>MSKATYKERAATHPSPVAAKLFNIMHEKQTNLCASLDVRTTKELLELVEALGPKICLLKTHVDILTDFSMEGTVKPL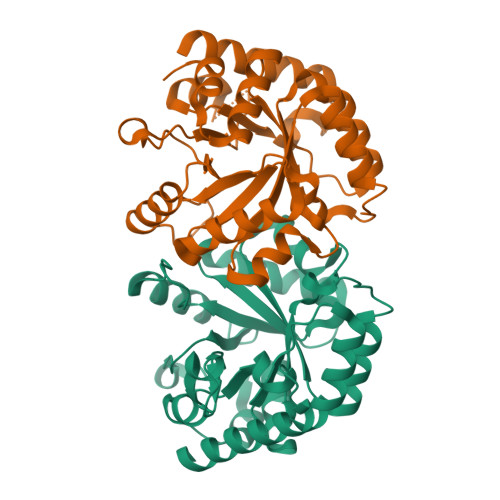KALSAKYNFLLFEDRRFADIGNTVKLQYSAGVYRIAEWADITNAHGVVGPGIVSGLKQAAEEVTKEPRGLLMLAELSCKGSLATGEYTKGTVDIAKSDKDFVIGFIAQRDMGGRDEGYDWLIMTPGVGLDDKGDALGQQYRTVDDVVSTGSDIIIVGRGLFAKGRDAKVEGERYRKAGWEAYLRRCGQQN[2x]> MAHHHHHHEFPKPEFMSKSLEELQIGTYANIAMVRTTTPVYVALGIFVQHRVSALPVVDEKGRV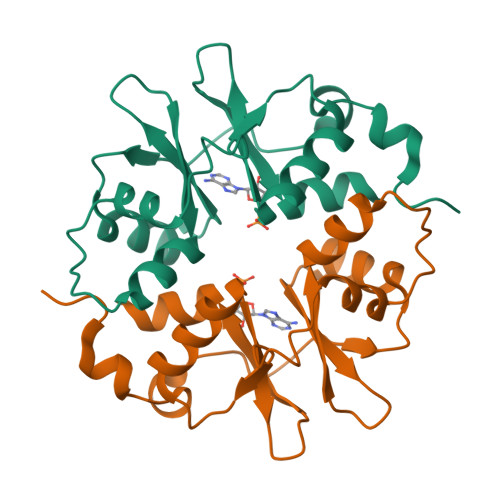VDIYSKFDVINLAAEKTYNNLDVSVTKALQHRSHYFEGVLKCYLHETLETIINRLVEAEVHGLVVVDENDVVKGIVSLSDILQALVLT> AETSSATTAQQMPSLAPMLEKVMPSVVSINVEGSTTVNTPRMPRNFQQFFGDDSPFCQEGSPFQSSPFCQGGQGGNGGGQQQKFMALGSGVIIDADKGYVVTNNHVVDNATVIKVQLSDGRKFDAKMVGKDPRSDIALIQIQNPKNLTAIKMADSDALRVGDYTVAIGNPFGLGETVTSGIVSALGRSGLNAENYENFIQTDAAINRGNSGGALVNLNGELIGINTAILAPDGGNIGIGFAIPSNMVKNLTSQMVEYGQVKRGELGIMGTELNSELAKAMKVDAQRGAFVSQVLPNSSAAKAGIKAGDVITSLNGKPISSFAALRAQVGTMPVGSKLTLGLLRDGKQVNVNLELQQSSQNQVDSSSIFNGIEGAEMSNKGKDQGVVVNNVKTGTPAAQIGLKKGDVIIGA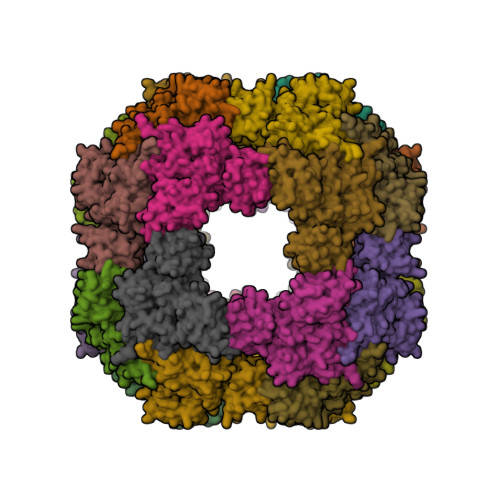NQQAVKNIAELRKVLDSKPSVLALNIQRGDSTIYLLMQRSHHHHHH>[12x]MTAPRSWAPTTRARGDTEALCSPEDGWVKVHPTPGTMLFREILHGQLGYTEGQGVYNVVRSSEATTRQLQAAIFHALLNATTYRDLEADWLGHVAARGLQPQR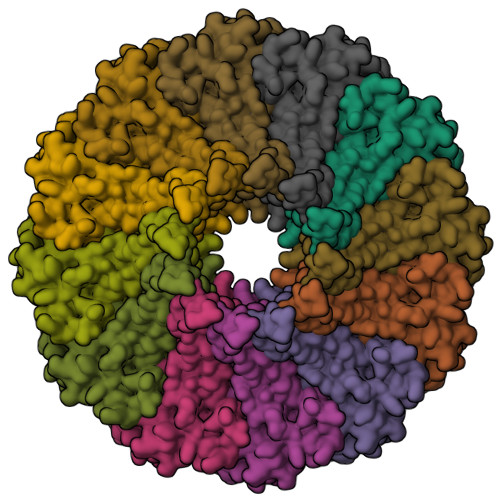LVRRYRNAREADIAGVAERVFDTWRNTLRTTLLDFAHGLVACFAPGGPSGPSSFPKYIDWLTCLGLVPILRKRQEGGVTQGLRAFLKQHPLTRQLATVAEAAERAGPGFFELALAFDSTRVADYDRVYIYYNHRRGDWLVRDPISGQRGECLVLWPPLWTGDRLVFDSPVQRLFPEIVACHSLREHAHVCRLRNTASVKVLLGRKSDSERGVAGAARVVNKVLGEDDETKAGSAASRLVRLIINMKGMRHVGDINDTVRAYLDEAGGHLIDAPAVDGTLPGFGKGGNSRGSAGQDQGGRAPQLRQAFRTAVVNNINGVLEGYINNLFGTIERLRETNAGLATQLQERDRELRRATAGALERQQRAADLAAESVTGGCGSRPAGADLLRADYDIIDVSKSMDDDTYVANSFQHPYIPSYAQDLERLSRLWEHELVRCFKILCHRNNQGQETSISYSSGAIAAFVAPYFESVLRAPRVGAPITGSDVILGEEELWDAVFKKTRLQTYLTDIAALFVADVQHAALPPPPSPVGADFRPGASPRGRSRSRSPGRTAPGAPDQGGGIGHRDGRRDGRR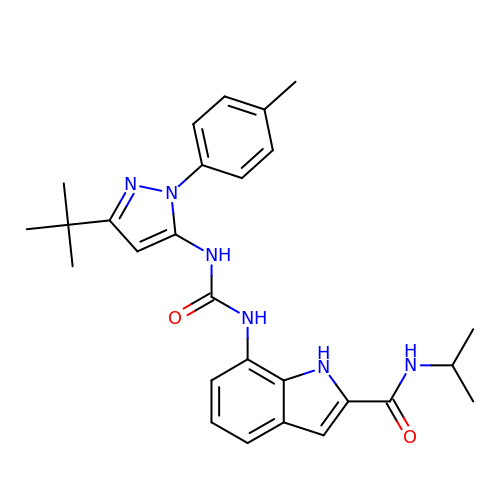7-({[3-tert-butyl-1-(4-methylphenyl)-1H-pyrazol-5-yl]carbamoyl}amino)-N-(propan-2-yl)-1H-indole-2-carboxamide | C27 H32 N6 O2 | WGABQSVUYBMTBW-UHFFFAOYSA-N> QAGFDLLNDGRPETLWLGIGTLLMLIGTFYFIARGWGVTDKEAREYYAITILVPGIASAAYLAMFFGIGVTEVELASGTVLDIYYARYADWLFTTPLLLLDLALLAKVDRVTIGTLIGVDALMIVTGLIGALSKTPLARYT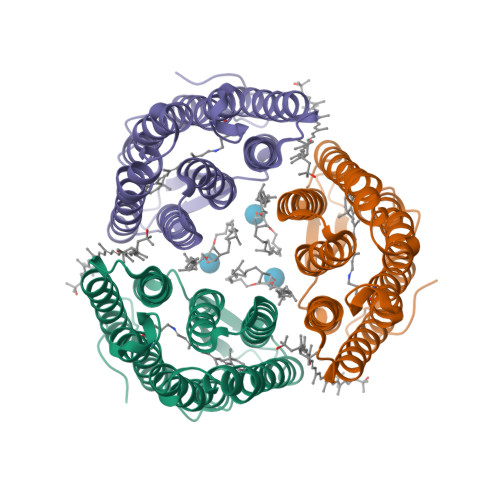WWLFSTIAFLFVLYYLLTSLRSAAAKRSEEVRSTFNTLTALVAVLWTAYPILWIVGTEGAGVVGLGIETLAFMVLDVTAKVGFGFVLLRSRAILGETEAPEPSAGADASAAD ethanedial | 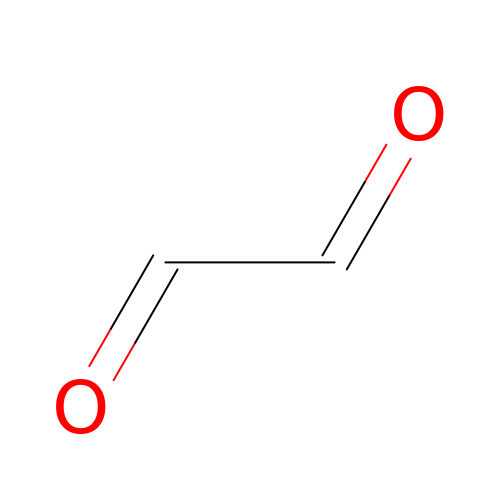C2 H2 O2 | LEQAOMBKQFMDFZ-UHFFFAOYSA-N Extracellular matrix binding protein (Embp) and its subdomains referred to as the F-repeat and the FG-repeat are critical for adherence of S. epidermidis to surface-immobilized Fn. Embp is a giant 1-MDa surface protein consisting of 10,203 amino acids (aa). High-resolution structure analysis of F- and FG-repeats revealed that both repeats are composed of two tightly connected triple α-helix bundles, exhibiting an elongated but rather rigid structural organization in solution. Both F- and FG-repeat possess Fn-binding capacity via interactions with type III subdomain FN12, involving residues within the C and F β-sheet.

The C-terminal repetitive region (aa 4511 to 9509), also present in S. aureus homolog Ebh, is composed by a row of 40 repeats consisting of 125 aa. This repeating unit is referred to here as the FG-repeat. Similar to the F-repeat, the FG-repeat reveals an elongated shape approximately 70 Å in length and 20 Å in width and height. A- and S-modules are connected by a shared helix α3, lancing through both three-helix bundles (the length of the central helix α3 is about 40 Å). The FG-repeat is characterized by a remarkable strong dipole character. The N-terminal region (A-module), formed by the N terminus of helix α1 and the N terminus of helix α3, is strongly positively charged, whereas the C-terminal region (S-module) formed by the C terminus of helix α6 and the short helix α4, is strongly negatively charged. Consistent with F-repeat analysis, the chemical similarity of each individual amino acid is low between individual FG-repeats, but the prediction of secondary structure features is well conserved. Although the overall amino acid sequence identity with Embp is only 30%, the structural data for the FG-repeat at 1.55-Å resolution reveals high structural homology to EbhA and strict conservation of all major structural key elements. Here, by strong interactions between subsequent FG-repeats, the dipole character of the FG-repeats likely supports the SAXS-deduced, elongated rod-like structure of repetitive FG-repeats. Importantly, the KD for rF-repeat binding to Fn was determined to be approximately 4.0 × 10−6 M, which is substantially higher compared to the KD value obtained for the rFG-repeat, i.e., 1.6 × 10−9 M.

> ADQKLQDAKTDAKQQITNFTGLTEPQKQALENIINQQTSRANVAKQLSHAKFLNGKMEELKVAVAKASLVRQNSNYINEDVSEKEAYEQAIAKGQEIINSENNPTISSTDINRTIQEINDAEQNLH> MS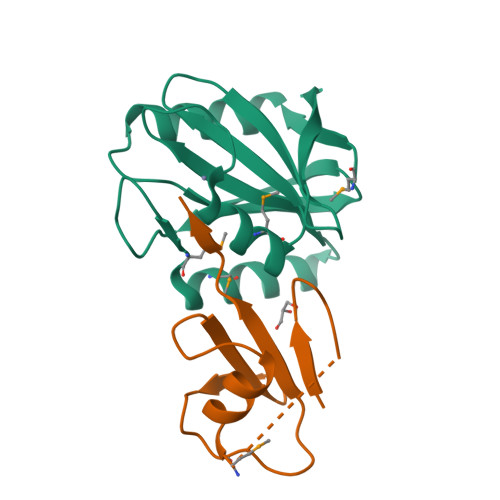TLIIPQHYLRAILKVVSSSSVEVCGFLFGKENRVLKVRFIRNRLNSPVEFEMDPEEMLKALEEAEQENLEVVGIFHSHIACPPIPSGKDLEGMKRWPVIWLIVNEKGEYKAWILSEKNKISEVKIVVE;> MKMIKVKVIGRNIEKEIEWREGMKVRDILRAVGFNTESAIAKVNGKVVLEDDEVKDGDFVEVIPVVSGG> GS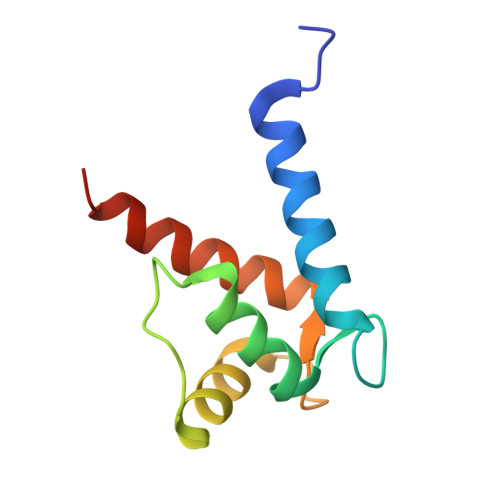HMSELEKAMVALIDVFHQYSGREGDKHKLKKSELKELINNELSHFLEEIKEQEVVDKVMETLDNDGDGECDFQEFMAFVAMVTTACHEFFEHE>[4x]MQTKHIAQATVKVLQSYLTYQAVL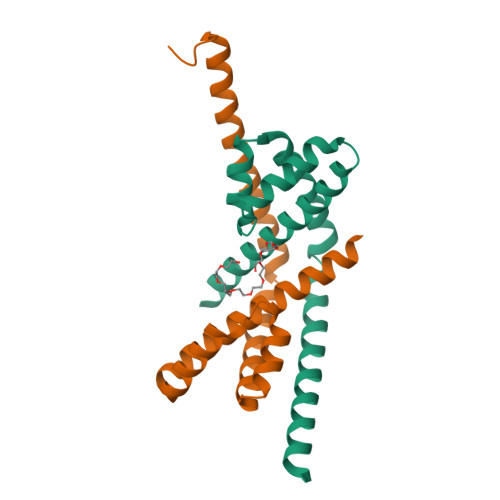RIQSELGETNPPQAIWLNQYLASHSIQNGETFLTELLDENKELVLRILAVREDIAESVLDFLPGMTRNSLAESNIAHRRHLLERLTRTVAEVDNFPSETSNGESNNNDSPPSAAALEHHHHHH>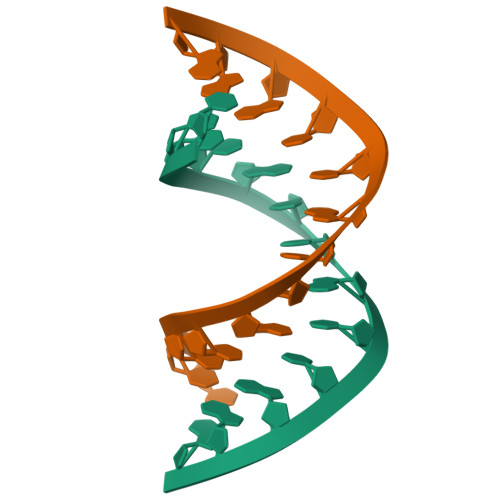 UUCUGCUGCUGAA>[2x]MNPTIIRARAPLR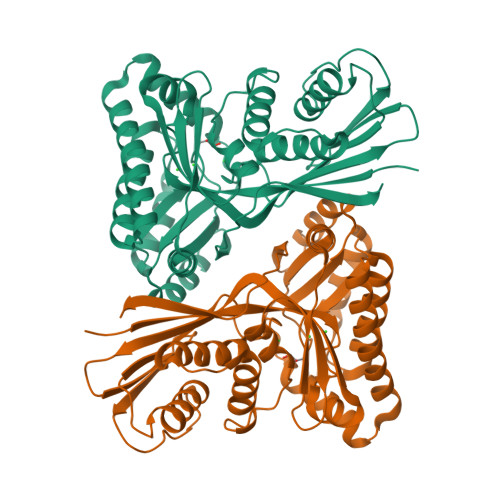LGLAGGGTDVAPYADTFGGYVLNATIDRYAYAVIKTLTIPAVRFVSTDQQVEKHQLISEPLELNGTLNLHKAVYNHMIRNYNHGKPIALELSTFCDAPAGSGLGSSSTLVVVMIKAFVELLNLPLDDYAIAQLAYRIERVDCGLAGGRQDQYSATFGGFNFMEFYEEERTIVNPLRIKNWVLCELEASLVLFYTGVSRESAKIIQDQSDNVVSHKTAAIEAMHGIKREALVMKEALLKGDFKAFVASMRLGWDNKKNSARTVSNAHIDEIYDAAIRAGAQAGKVSGAGGGGFMLFFVPTEKRMDLIRTLGEYDGQVSNCHFTKNGTQAWRIAN>[2x]FHTVDVK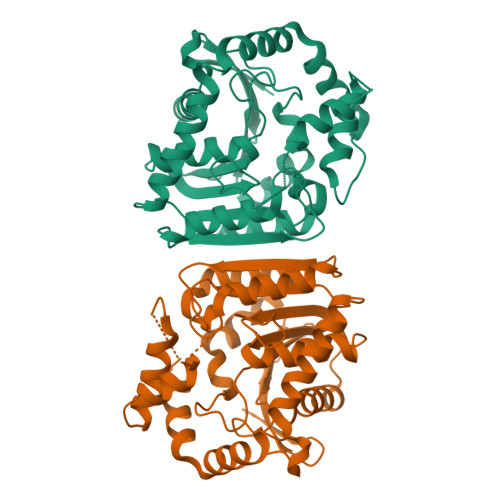GVQTRYFDDGQDKDPILLIHGGHFGFFIPVGIESWGNVLEDFGEYGRVLAVDKLGQGETGLPLNDEDWTVDAVAEHVANFATQLGLKNLTLVGHSRGGMTAVLLALKYPEMVKKLVIISSATAAPAPPVGTDMDFYERVERTAPGGSAELIRHYHAAQAVNEGDLPEDYIGIATKWLESEKQLDAVAGYARNAEEHWLPSLSEGRRWVQERLADAGIPVPTLVVWGVNDRSAPVSMGKGLFDLIAANTLDSSLYLINNAGHHVFSDQREKFNAAVGAFISL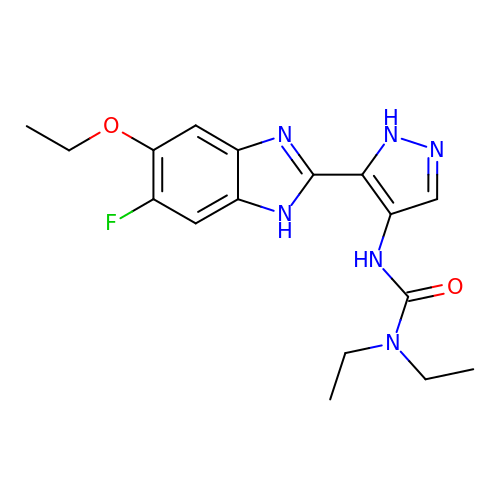3-[5-(5-ethoxy-6-fluoro-1H-benzimidazol-2-yl)-1H-pyrazol-4-yl]-1,1-diethylurea | C17 H21 F N6 O2 | UJXIKUVGGQECLJ-UHFFFAOYSA-N(5E)-5-[(2,2-DIFLUORO-1,3-BENZODIOXOL-5-YL)METHYLENE]-1,3-THIAZOLIDINE-2,4-DIONE | C11 H5 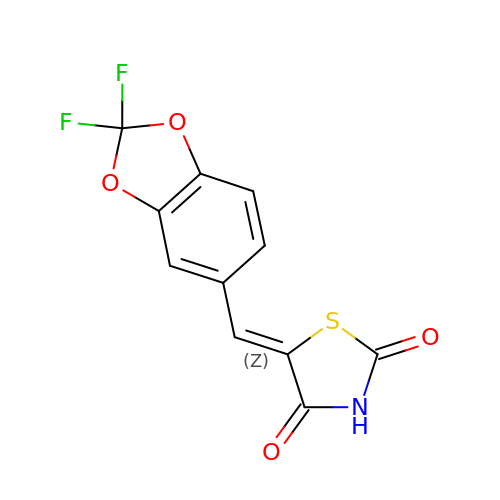F2 N O4 S | SRLVNYDXMUGOFI-YWEYNIOJSA-N>MASNSPTFKHESYYATVNELTPVGTTIFTGFSGDNGATDIDDGPNGQIEYVIQYNPDDPTSNDTFEIPLMLTGNIVLRKRLNYEDKTRYFVIIQANDRAQNLNERRTT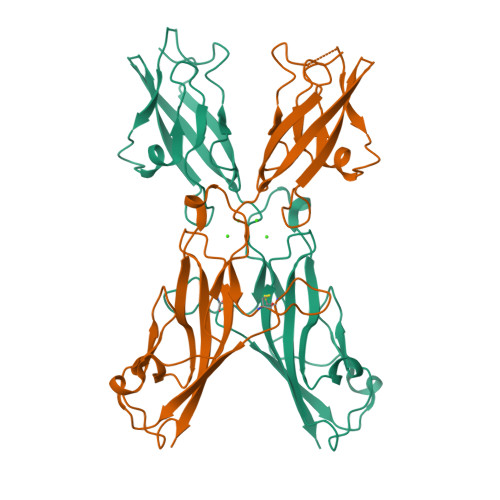TTTLTVDVLDGDDLGPMFLPCVLVPNTRDCRPLTYQAAIPELRTPEELNPIIVTPPIQAIDQDRNIQPPSDRPGILYSILVGTPEDYPRFFHMHPRTAELSLLEPVNRDFHQKFDLVIKAEQDNGHPLPAFAGLHIEILDENNLEHHHHHH[4x]(2-BROMOETHYL)(2-'FORMYL-4'-AMINOPHENYL) 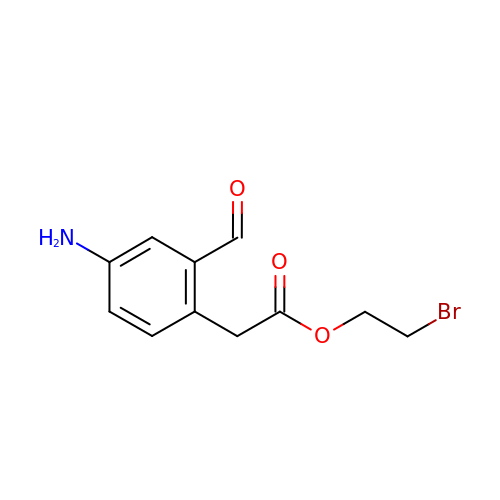ACETATE | C11 H12 Br N O3 | SMKXVWWBCFWRMP-UHFFFAOYSA-N>HHHHHHGSSQLLPAPLTNDPTAIGPVLPFEELHPRRYPENTATFLTRLRSLPSNHLPQPTLNCLLSAVSDQTKVSEEHLWESLQTILPDSQLSNEETNTLGLSTEHLTALAHLYNFQATVYSDRGPALF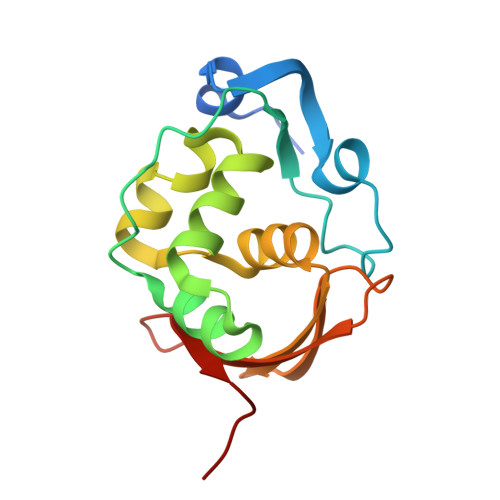GPSDTIKRIDITHTTGPPSHFSPGKRLLGS[2x]>[2x]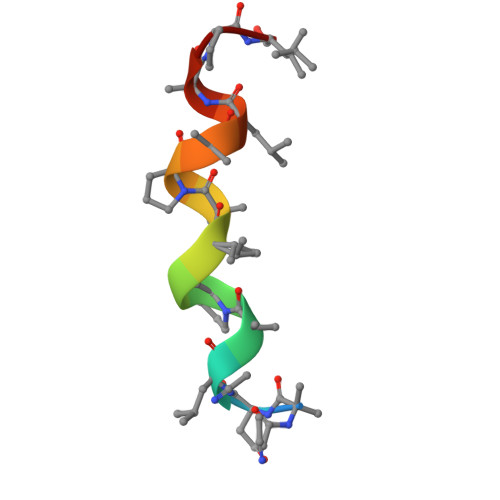XANLAPAVAPALAPX>[2x]GSALEKVPVEEYLVHALQGSVSSGQAHSLASLAKTWSSGSAKLQRLGPETEDNEGVLLTEKLKPVDYEYREEVHWMTHQPRVGRGSFGEVHRMKDKQTGFQCAVKKVRLEVFRVEELVACAGLSSPRIVPLYGAVREGPWVNIFMELLEGG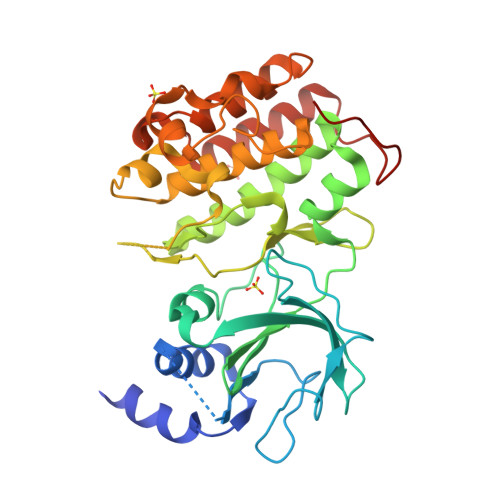SLGQLIKQMGCLPEDRALYYLGQALEGLEYLHTRRILHGDVKADNVLLSSDGSRAALCDFGHALCLQPDGLGKSLLTGDYIPGTETHMAPEVVMGKPCDAKVDIWSSCCMMLHMLNGCHPWTQYFRGPLCLKIASEPPPIREIPPSCAPLTAQAIQEGLRKEPVHRASAMELRRKVGKALQEVGGLKSPWKGEYKEPRGNS> ADTIVAVELDTYPNTDIGDPSYPHIGIDIKSVRSKKTAKWNMQNGKVGTAHIIYNSVGKRLSAVVSYPNGDSATVSYDVDLDNVLPEWVRVGLSASTGLYKETNTILSWSFTSKLKSNSTHETNALHFSFNQFSKDQKDLILQGDATTGTDGNLELTRVSSNGSPQGSSVGRALFYAPVHIWESSAVVASFDATFTFLIKSSDSHPADGIAFFI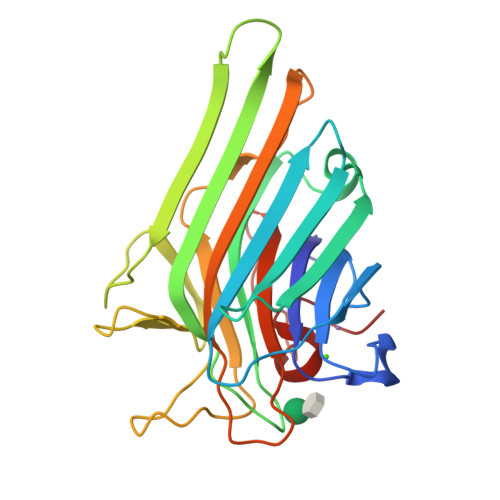SNIDSSIPSGSTGRLLGLFPDAN methyl N-[(5Z)-6-({[4-(4-iodobenzyl)phenyl]carbonyl}amino)hex-5-enoyl]glycinate 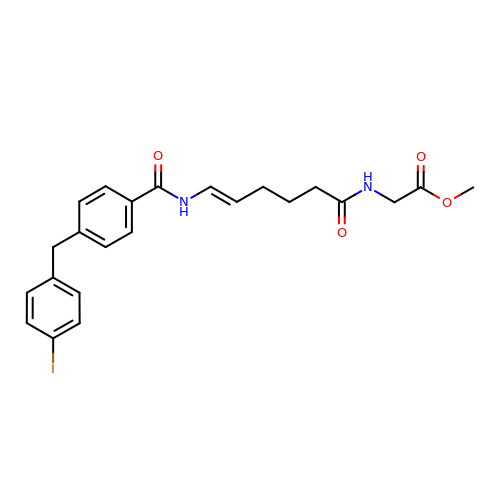| C23 H25 I N2 O4 | GJXNVOLPXGNHOU-CPSFFCFKSA-N> MEQKQQSERLGTEAIPKLLRSLSIPAMIGMFVMALYNVVNTIFISYAVGIEGVAGVTIAFPIMMIMMSMAGALGIGGASVISRRLGERRGEEANQVFGNILTVILVLSVIGFISAFTLLGPALQLFGATSVTQGYATDYLFPILLGSIFFFFAFAANNIIRSEGNATFAMVTMIVPAVLNILLDVLFIFGLNMGVLGASIATVIAQASVTGLVLRYFLTGKSTLSLHWSDLRMKGSVIKEVCLVGLPAFVQQSSASLMMIAINSMLLRFGSDFYVGVFGLVQRIMMFVMMPMMGIMQAMQPIVGYNYGAKQYSRLRETVMLGFKVATIFSIGIFALLMLFPEALLRVFTADREVIQAGVSAMHILFCVTFLIGAQIVAGGLYQSLGKPKQALILSLSRQIIFLIPLVLILPHIFGLSGVWWAFPIADVLSFILTVVLLYRDRNVFFLKTKEERELDLVKTASS

Integral membrane proteins belonging to the multidrug and toxic compound extrusion (MATE) family contribute to multidrug resistance by using either the Na+ or H+ electrochemical gradient to extrude drugs across cell membranes. MATE proteins identified thus far can be separated into the NorM, DinF and eukaryotic subfamilies based on amino-acid sequence similarity. Those crystal structures revealed a similar protein fold comprising 12 membrane-spanning segments (TM1-TM12), they nevertheless suggested different arrangement of cation- and substrate-binding sites between the NorM and DinF proteins, hinting at substantial mechanistic diversity among the MATE transporters.

We replaced DinF-BHD40 with asparagine, mimicking a constitutively protonated aspartate. This mutation abrogated the transport function9, likely because the protein was trapped in a protonated state. We also soaked DinF-BHD40N crystals into low pH (∼4) solutions, and determined the structure to 3.0 Å resolution by combining molecular replacement and MIRAS phasing. The low pH-soaked structure of DinF-BHD40N is largely identical to the un-soaked one (root mean squared deviation (r.m.s.d.) <0.5 Å for 447 Cα positions), ascertaining that the protein was indeed locked into a protonated state. Tellingly, TM1 in DinF-BHD40N is no more bent than that of DinF-BH, suggesting the notion that TM1 is kinked in an extracellular-facing, protonated MATE transporter is not always applicable. The most functionally important difference involves the side chain of DinF-BHD40N, which participates in an H-bonding network also involving DinF-BHY36 (TM1), DinF-BHN180, DinF-BHD184 (TM5) and DinF-BHT202 (TM6). In this network, the side chain of DinF-BHD40N forms an H-bond with that of DinF-BHD184. By contrast, in the deprotonated DinF-BH9, no such interaction was observed between DinF-BHD40 and DinF-BHD184. Taken together, we suggest that H+ evokes substrate release by breaking the charge–charge interaction between the deprotonated DinF-BHD40 and the bound substrate, and by engaging the protonated DinF-BHD40 in an H-bonding interaction with DinF-BHD184. Our results suggested that the protonation of TM1 in DinF-BH induces the release of substrate without entailing significant structural changes in the extracellular-facing transporter, including the bending of TM1.>ADTIVAVELDTYPNTDIGDPSYPHIGIDIKSVRSKKTAKWNMQNGKVGTAHIIYNSVDKRLSAVVSYPNADSA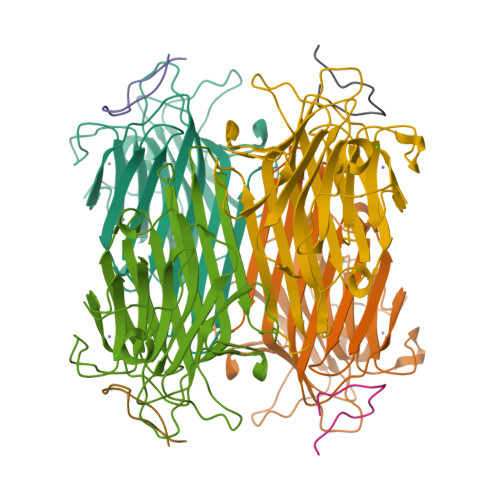TVSYDVDLDNVLPEWVRVGLSASTGLYKETNTILSWSFTSKLKSNSTHETNALHFMFNQFSKDQKDLILQGDATTGTDGNLELTRVSSNGSPQGSSVGRALFYAPVHIWESSAVVASFEATFTFLIKSPDSHPADGIAFFISNIDSSIPSGSTGRLLGLFPDAN[4x];>[4x]RVWYPYGSYLTASGS N~5~-[2-(methylsulfanyl)ethanimidoyl]-L-ornithine | C8 H17 N3 O2 S | 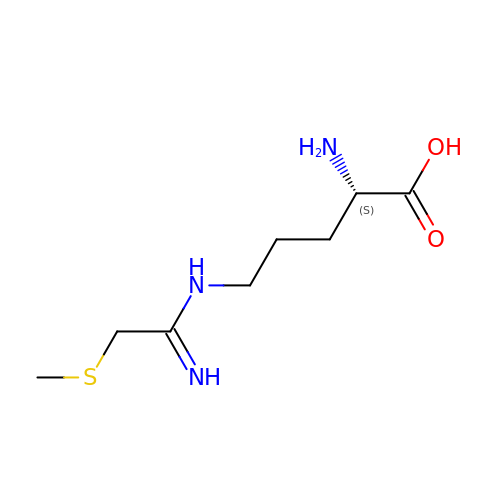VXQPBNRYLWZLLJ-LURJTMIESA-N>ELICIVQRVNESFSLHSGFGGNVYSMKTEPMTGFTNVTKGASVINQKDWIGFGDARTDLTNDQFPASSDVPLAVAKKFRSLSGASLMLSAFGPPGKVDYLYQGCGKE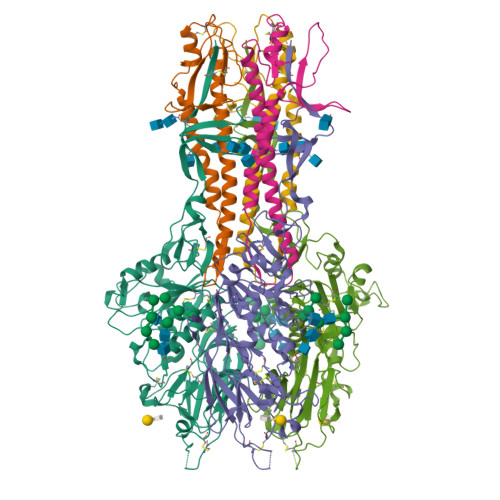KVFYEGVNWSPEAGIDCFGSNWTQTKKDFYSRIYEAARSSTCMTLVNSLDTKISSTTATAGTASSCSSSWMKSPLWYAESSVNPGAKPQVCGTEQSATFTLPTSFGIYKCNKHVVQLCYFVYENKAKFNTFGCGDYYQNYYDGNGNLIGGMDNRVAAYRGIANAGVKIECPSKILNPGTYSIKSTPRFLLVPKRSYCFDTDGGYPIQVVQSEWSASRRSDNATEEACLQTEGCIFIKKTTPYVGEAADNAGDIEMRQLLSGLGNNDTVCVSQSGYTKGETPFVKDYLSPPKYGRCQLKTDSGRIPTLPSGLIIPQAGTDS[2x];>[2x]IFGIDDLIFGLLFVGFVAGGVAGGYFWGRSNGGGGGASVSSTQAGFDKIGKDIQQLRNDTNAAIEGFNGRIAHDEQAIKNLAKEIEDARAEALVGELGIIRSLIVANISMNLKESLYELANQITKRGGGIAQEAGPGCWYVDSENCDASCKEYIFNFNGSATVPTL6-azanyl-2-[[(1~{R},2~{S},6~{S},9~{R})-4,4,11,11-tetramethyl-3,5,7,10,12-pentaoxatricyclo[7.3.0.0^{2,6}]dodecan-6-yl]methylamino]-3,7-dihydroimidazo[4,5-g]quinazolin-8-one 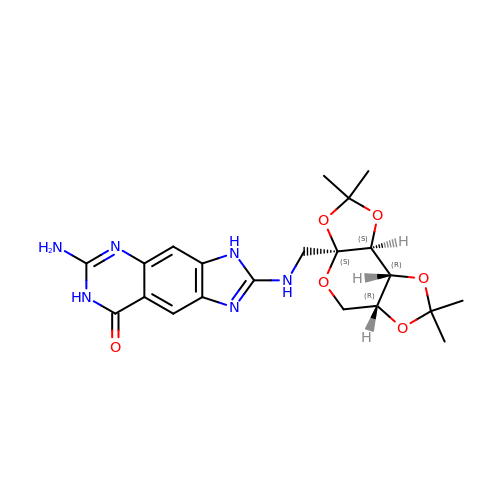| C21 H26 N6 O6 | DBANTQMQBSPBCW-MBIULKOWSA-N Peroxiredoxins scavenge ROS via their peroxidase activity, reducing hydrogen peroxide and a wide range of organic hydroperoxides. PRDX1 is a crucial antioxidant protein to regulate oxidative stress. Then peroxiredoxin 1 (PRDX1) was identified as the ROS-manipulating target protein of Celastrol in colorectal cancer. To obtain homogeneous oligomeric and less flexible proteins for crystallization, the Cys-52 and Cys-83 residues were mutated to serine, and the C-tail of PRDX1 (176-199 aa) was truncated.

To reveal the stereospecific conjugation and binding mode of Celastrol, the crystal structure of PRDX1 in complex with Celastrol was solved to the resolution of 1.76 Å. Then it was found that two PRDX1C52SC83S,1-175aa monomers formed a head-to-tail homodimer, and two Celastrol molecules were covalently linked to the Cys-173 residues of the homodimer. Moreover, the 2Fo-Fc electron density map contoured to 1.0σ for Celastrol linked to the Cys-173 residues confirms that Celastrol is a covalent inhibitor of PRDX1. For each PRDX1C52SC83S,1-175aa homodimer, the covalently linked two Celastrol molecules stretched into and formed non-covalent interactions with adjacent homodimers. Interestingly, the binding modes of two Celastrol molecules with adjacent PRDX1 homodimers are different. For one Celastrol molecule, direct and water-bridged hydrogen bonds were observed with the Trp-87, Asn-89, Gln-94 residues of adjacent PRDX1 homodimer. While for another Celastrol molecule, direct and water-bridged hydrogen bonds were observed with the Arg-140, Thr-166, His-169 residues of another adjacent PRDX1 homodimer. For one Celastrol molecule, hydrophobic contacts were formed with the Phe-48 and Val-172 residues, while for another Celastrol molecule, less hydrophobic contacts were observed. The covalent binding residue (Cys-173) and non-covalent binding residues are from different PRDX1 homodimers. It is known that PRDX1 homodimers form into decamers in its catalytic cycle, then this unique binding mode of Celastrol with PRDX1 homodimers is likely to disrupt the decamer formation of PRDX1 homodimers.

>MSSGNAKIGHPAPNFKATAVMPDGQFKDISLSDYKGKYVVFFFYPLDFTFVSPTEIIAFSDRAEEFKKLNCQVIGASVDSHFSHLAWVNTPKKQGGLGPMNIPLVSDPKRTIAQDYGVLKADEGISFRGLFIIDDKGILRQITVNDLPVGRSVDETLRLVQAFQFTDKHGEVCPA[2x]> GDVVEAVENAVARVADTIGSGPSNSQAVPALTAVETGHTSQVTPSDTVQTRHVKNYHSRSESSIENFLSRSACVYMGEYHTTNSDQTKLFASWTISARRMVQMRRKLEIFTYVRFDVEVTFVITSKQDQGTQLGQDMPPLTHQIMYIPPGGPIPKSVTDYTWQTSTNPSIF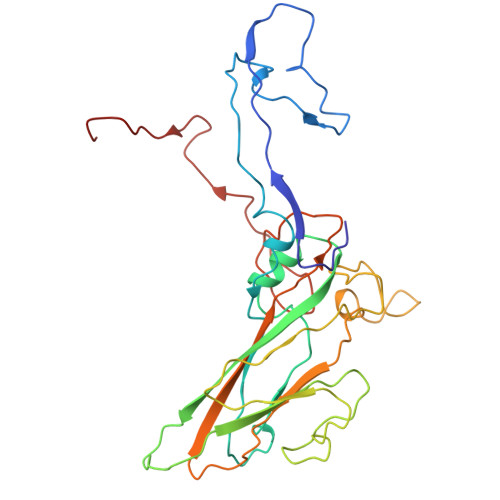WTEGNAPPRMSIPFISIGNAYSNFYDGWSHFSQNGVYGYNTLNHMGQIYVRHVNGSSPLPMTSTVRMYFKPKHVKAWVPRPPRLCQYKNASTVNFSPTDITDKRNSITYIPDTVKPDV> GSRKIIHVDMDCFAAAVEMRDNPALRDIPIAIGGSRERRGVISCANYPARKFGVRSAMPTGMALKLCPHLTLLPGRFDAYKEASNHIREIFSRYTSRIEPLSLDEAYLDVTDSVHCHGSATLIAQEIRQTIFNE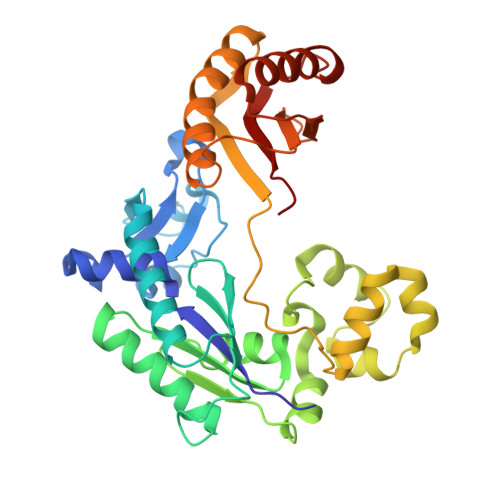LQLTASAGVAPVKFLAKIASDMNKPNGQFVITPAEVPAFLQTLPLAKIPGVGKVSAAKLEAMGLRTCGDVQKCDLVMLLKRFGKFGRILWERSQGIDERDVNSERLRKSVGVERTMAEDIHHWSECEAIIERLYPELERRLAKVKPDLLIARQGVKLKFDDFQQTTQEHVWPRLNKADLIATARKTWDERRGGRGVRLVGLHVTLLDP> TNLVAEPFAKLEQDFGGSIGVYAMDTGSGATVSYRAEERFPLCSSFKGFLAAAVLARSQQQAGLLDTPIRYGKNALVPWSPISEKYLTTGMTVAELSAAAVQYSDNAAANLLLKELGGPAGLTAFMRSIGDTTFRLDRWELELNSAIPGDARDTSSPRAVTESLQKLTLGSAL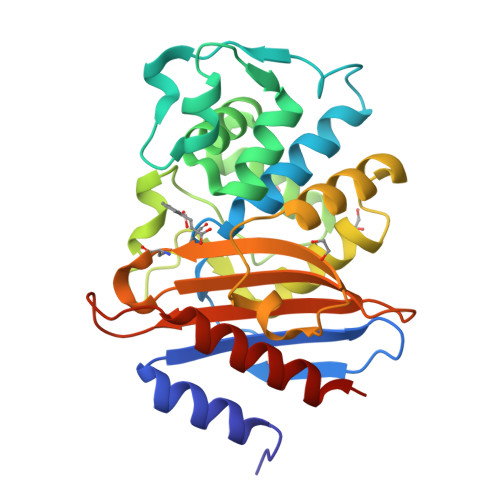AAPQRQQFVDWLKGNTTGNHRIRAAVPADWAVGDKTGTCGVYGTANDYAVVWPTGRAPIVLAVYTRAPNKDDKHSEAVIAAAARLALEGLGVNGQ>MTTPISPPPQWSRRRQEKQRRLERVRGLADGAVLPREGLVAALEALIAPGDRVVLEGNNQKQADFLSRSLARVDPGKLHDLHMIMPSVGRPEHLDLFELGIARKLDFSFSGPQSLRIGQLLEDGLLEIGAIHTYIELYARLVVDLIPNVALVAGFVADREGNVYTGPSTEDTPALVEPTAFSDGIVIVQVNRIVDDPRDLPRVDIPASWVDFVVEADQPFYIEPLFTRDPRHIKPVHVLMAMMAIRGIYQRHNVQSLNHGIGFNTAAIELILPTYGESLGLKGKICRHWTLNPHPTLIPAIESGWVESVHCFGTELGMEGYIAQRPDVFFTGRDGSLRSNRMFCQLAGQYAVDLFIGATLQVDGDGHSSTVTRGRLAGFGGAPNMGHDPRGRRHSTPAWLDMRGEPEALLERGRKLVVQMVETFQDGGKPTFVERLDALEVARQTGMPLAPVMIYGDDVTHVLTEEGIAYLYKARSLEERQAMIAAVAGISPIGLRHDPRETQRMRREGLIALPEDLGIRRTDASRELLAAKSIAELVEWSGGLYQPPARFRSW[2x];>METLSFEFPAGQPGRGRALVGCVGSGDLEVLLEPGQPGKLSIQVQTSVNGSASRWQHLFERLFDGQTPPALLIDIHDFGATPGVVRLRLEQGFEEIGHD[2x];>MTDVARLLALRSFTELGARQRARALLDAGSFRELLDPFAGVQSPWLERQGIVPQADDGVVVARGLLDGQPAVLAAIEGAFQGGSLGEVSGAKIAGALELAAEDNRNGVPTRALLLLETGGVRLQEANLGLAAIAEIQAAIVDLQRYQPVVAVIAGPVGCFGGMSIAAGLCSYVLVTREARLGLNGPQVIEQEAGIAEYDSRDRPFIWSLTGGEQRFASGLADAYLADDLDEVRTSVLAYFAKGLPARPRCRRAEDYLRRLGDLDTAEQPDAAGVRRLYQGLGQGDAT[2x];>MGSSHHHHHHSQDPNSMSQPFASRGLAWFQALAGSLAPRPGDPASLRVADAELDGYPVRFLAVVPDPDNPFPRARQGEVGLLEGWGLAAAVDEALEADREAPRKRALLAIVDVPSQAYGRREEALGIHQALAGAVDAYARARLAGHPLIGLLVGKAMSGAFLAHGYQANRLIALHDPGVMVHAMGK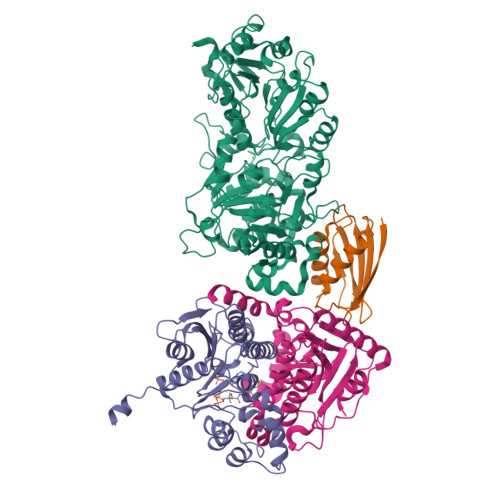AAAARITLRSVEELEALAAKVPPMAYDIDSYASLGLLWRTLPVETVEVPSTADLVRVRTCLGEALADILGGPRDLGGRLGAANREASARVRRLLREQW[2x]>[3x]MVNNNRPRRQRAQRVVVTTTQTAPVPQQNVPRNGRRRRNRTRRNRRRVR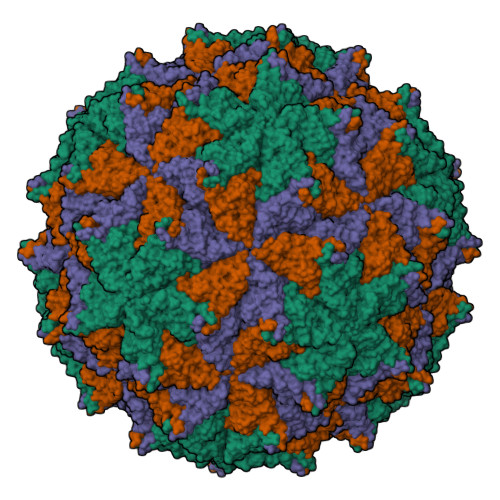GMNMAALTRLSQPGLAFLKCAFAPPNFNTDPGKGIPDRFEGKVVSRKDVLNQSISFTAGQDTFILIAPTPGVAYWSASVPAGTFPTSATTFNPVNYPGFTSMFGTTSTSRSDQVSSFRYASMNVGIYPTSNLMQFAGSITVWKCPVKLSTVQFPVATDPATSSLVHTLVGLDGVLAVGPDNFSESFIKGVFSQSACNEPDFEFNDILEGIQTLPPANVSLGSTGQPFTMDSGAEATSGVVGWGNMDTIVIRVSAPEGAVNSAILKAWSCIEYRPNPNAMLYQFGHDSPPLDEVALQEYRTVARSLPVAVIAAQNASMWERVKSIIKSSLAAASNIPGPIGVAASGISGLSALFEGFGF> DCGQPRNLPNGDFRYTTTMGVNTYKARIQYYCHEPYYKMQTRAGSRESEQGVYTCTAQGIWKNEQKGEKIPRCLPVCGKPVNPVEQRQRIIGGQKAKMGNFPWQVFTNIHGRGGGALLGDRWILTAAHTLYPKEHEAQSNASLDVFLGHTNVEELMKLGNHPIRRVSVHPDYRQDESYNFEGDIALLELENSVTLGPNLLPICLPDNDTFYDLGLMGYVSGFGVMEEKIAHDLRFVRLPVANPQACENWLRGKNRMDVFSQNMFCAGHPSLKQDACQGDSGGVFAVRDPNTDRWVAT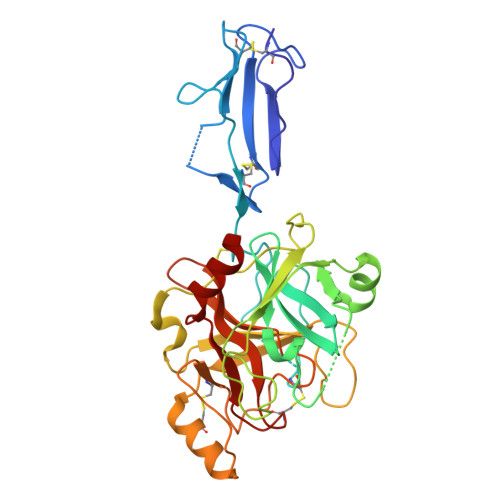GIVSWGIGCSRGYGFYTKVLNYVDWIKKEMEE> MGTRDDEYDYLFKV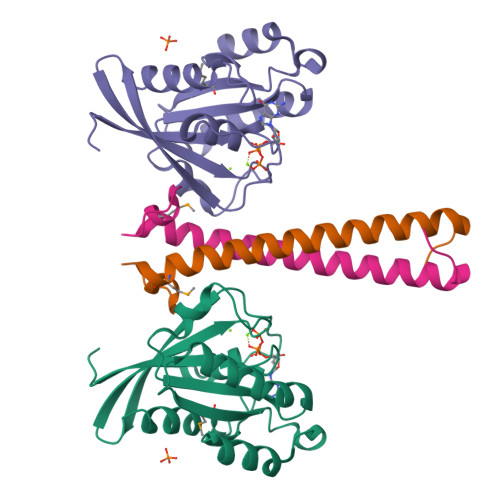VLIGDSGVGKSNLLSRFTRNEFNLESKSTIGVEFATRSIQVDGKTIKAQIWDTAGLERYRAITSAYYRGAVGALLVYDIAKHLTYENVERWLKELRDHADSNIVIMLVGNKSDLRHLRAVPTDEARAFAEKNGLSFIETSALDSTNVEAAFQTILTEIY;> GAMAAKFRASNIMPSSSFHMSPTSNEDLRKIPDSNPFDATAGYRSLTYEEVLQELVKHKELLRRKDTHIRELEDYIDNLLVRVMEETPSILRVPYEPSRKAGKFSNS PHENYL(SULFO)ACETIC ACID | C8 H8 O5 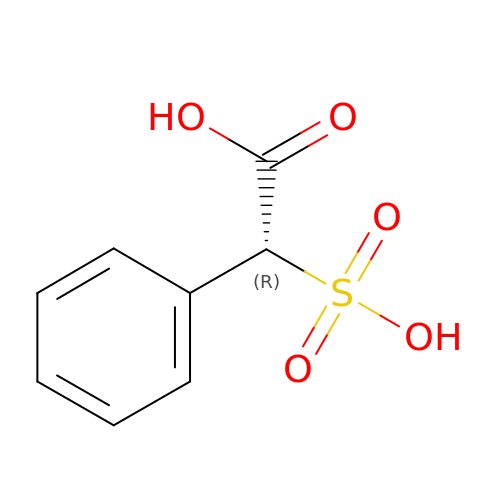S | USNMCXDGQQVYSW-SSDOTTSWSA-N> EVVGGGDLGPNVLVFDPSTPDIQGKVDEVFRKQESNQFGTDRYALMFKPGTYNDINAQIGFYTSIAGLGLNPDDTTFNGDVTVDAGWFDGNATQNFWRSAENLALNPVNGTNRWAVSQAAPFRRMHVKGGLNLAPDGYGWASGGYIADSKIDGEVGPYSQQQWYTRDSSVGGWGNGVWNMTFSGVEGAPAQSFPEPPYTTLETTPVSREKPFLYLDGDDYKVFVPAKRTNARGTSWGNGTPEGESLPLDQFYVVKPGATAETINAAVDQGLHLLFTPGVYHVDQPIEIDRANTVALGLGLATIIPDNGVTALKVGDVDGVKVAGLLVDAGPVN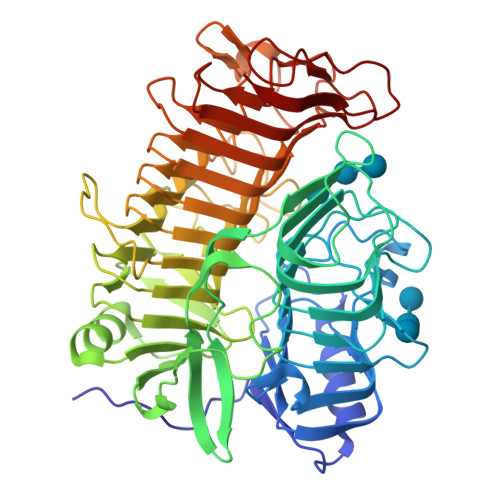SETLVEVGSDGASGDHAANPTSLQDVFVRIGGAGPGKATTSIVVNSNDTIIDHTWVWRADHGEGVGWETNRADYGVHVKGDNVLATGLFVEHFNKYDVQWSGENGKTIFYQNAKAYDAPDQAAIQNGDIKGYAAYKVDDSVTTHEGWGMGSYCYFNVNPDIRQQHGFQAPVKPGVKFHDLLVVSLGGKGQYEHVINDIGDPTSGDTTIPSQVVSFP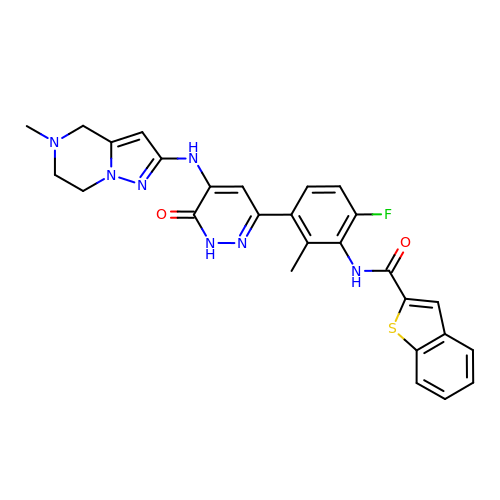N-(6-fluoro-2-methyl-3-{5-[(5-methyl-4,5,6,7-tetrahydropyrazolo[1,5-a]pyrazin-2-yl)amino]-6-oxo-1,6-dihydropyridazin-3-yl}phenyl)-1-benzothiophene-2-carboxamide | C27 H24 F N7 O2 S | MZSDTUIZKGUVHK-UHFFFAOYSA-N> GPAMVEVPRNFRLLEELETGEKGTGSNQNVSVGLRDTADIFFHYWNGTIVGPPSTTFEYRILSLEIYCDENYPKVPPHIRFLSKVNLPCVDSDGTVNREKFHVFKHWDRRTTMELC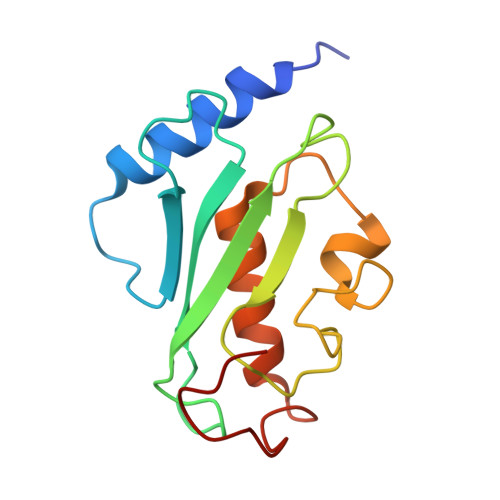LSELRKEMAQPQNRKLVQPPEGSTY>[4x]MGSSHHHHHHSSRNLYFQGGGHMFFLNLKQINDRFNTEFITKFKEILESGWYILGKQCEKFENNFAKYCGVKHCIGVANGLDALRLIIKAYDFKENDEIIVPANTYIASILAITDNKCKPILIEPDINTYNINPDLIEEKITKKTKAIMVVHLYGQVCDMEKIQLLANKYNLKIIEDCAQAHGAIYKDKRVGNLGDAAGFSFYPGKNLGALG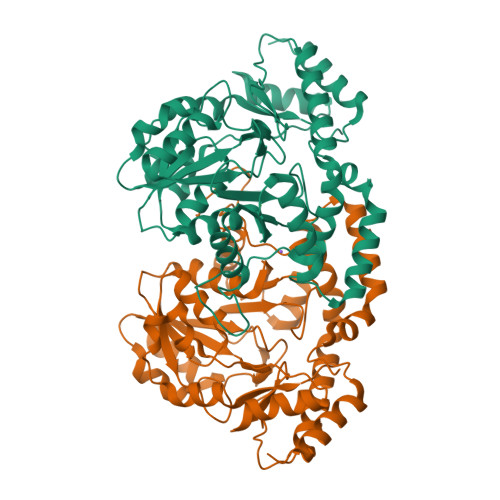DAGCICTNDDNFASKIRALANYGSHKKYENLYTGLNSRLDEIQAAFLDIKLKYLDEDNNKRKNIANFYLQNIKNENIILPSNKFDHVWHLFVVKTKLRDELQHYLNNHDIQTIIHYPIPPHKQKCYKDLNHLKLPITENIHQEVLSLPISPTMKENDFKKVADILNKWKV> GSAMGMSNTQAERSIIGMIDMFHKYTGRDGKIEKPSLLTMMKENFPNFLSACDKKGIHYLATVFEKKDKNEDKKIDFSEFLSLLGDIAADYHKQSHGAAPCSGGSQAAA

S100 proteins are a family of small, EF-hand containing calcium-binding signaling proteins that are implicated in many cancers. Hallmarks of the S100 protein family include their small size (~ 100 aa) and the presence of a canonical (calmodulin-like) EF-hand motif and a non-canonical (S100-specific) EF-hand motif. While most S100 proteins share moderate sequence identity, S100A7 and S100A15 are 93% identical in sequence yet intriguingly display divergent functions. Intriguingly, however, S100A7 and S100A15 serve distinct roles in inflammatory skin disease; S100A7 signals through the receptor for advanced glycation products (RAGE) in a zinc-dependent manner, while S100A15 signals through a yet unidentified G-protein coupled receptor in a zinc-independent manner.

Similar to S100A7, S100A15 eluted as a stable dimer from a size exclusion column (SEC) indicating that the seven divergent residues (R21GD24GD27ET83AT51IN52H and D56T – S100A7 residues are shown in italics and S100A15 residues are underlined) did not disrupt the multimeric structure. S100A15 crystallized as a monomer in the asymmetric unit of the monoclinic cell with the dimer generated by crystallographic symmetry. The S100A15 structure was refined to a resolution of 1.7 Å and displayed an overall root mean squared deviation (r.m.s.d) of 0.661 Å2 over 96 Cα atoms relative to S100A7. During the initial refinement stages of the S100A15 structure an 8 sigma difference electron density peak was observed that overlaid with the bound zinc in S100A7. Accordingly, a zinc ion was modeled and refined at full occupancy resulting in a B-factor of 30.52 Å2. Thus, it was apparent that substitution of Gly24 in S100A15 for the zinc ligand Asp24 (S100A7) did not abrogate zinc binding. To complete the distorted tetrahedral geometry of the bound zinc in S100A15, a chloride ion was modeled, which refined to a distance of 2.1 Å from the zinc and a B factor of 25.4 Å2. While water molecules are commonly observed as labile ligands in zinc coordination sites, we elected to model a chloride ion using the B factor as a guide and based on the fact that chloride was the dominant anion in our buffer. A second zinc atom was observed in the S100A15 structure (at Glu36), which was not observed in the S100A7D24G mutant. We expect this is an artifact as S100A15 WT was crystallized in high concentrations (50 mM) of zinc while S100A7D24G was crystallized in the absence of zinc.> GP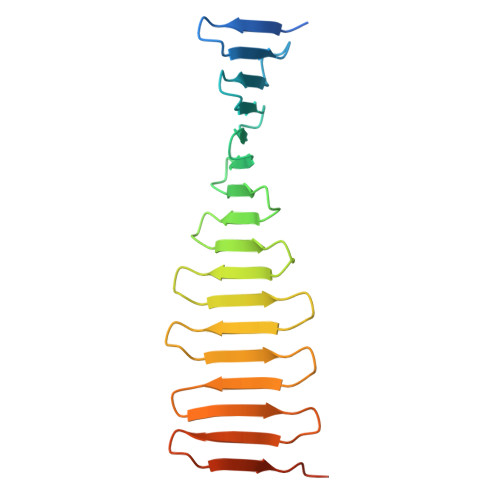LGSDSKIEKMLPDGGRLVVFPNGTRKELSADGQTVKVMFFNGDVKHTMPDQRVIYYYAEAQTTHITYPDGMEVLQFPNNQTEKHFPDGRKEITFPDQTVKTLHPDGREESVLTDGTIIQLNPDGSKVIQFNTGQREIHTADFKRREYPDGTVKTVYSDGRQETQYPTGRVRLKDPQGKVIMD> MNINDNLSINSPVDNKNVVVVRARKTDTVFKAFKVAPNIWVAPERYYGESLSIDEEYKVDGGIYDSNFLSQDSEKDKFLQAIITLLKRINSTNAGEKLLSLISTAIPFPYGYIGGGYYAPNMITFGSAPKSNKKLNSLISSTIPFPYAGYRETNYLSSEDNKSFYASNIVIFGPGANIVENNTVFYKKEDAENGMGTMTEIWFQPFLTYKYDEFYIDPAIELIKCLIKSLYFLYGIKPSDDLVIPYRLRSELENIEYSQLNIVDLLVSGGIDPKFINTDPYWFTDNYFSNAKKVFEDHRNIYETQIEGNNAIGNDIKLRLKQKFRININDIWELNLNYFSKEFSIMMPDRFNNALKHFYRKQYYKIDYPENYSINGFVNGQINVQLSLSDRNQDIINKPEEIINLLNGNNVSLMRSNIYGDGLKSTVDDFYSNYKIPYNRAYEYHFNNSNDSSLDNVNIGVIDNIPEIIDVNPYKENCDKFSPVQKITSTREINTNIPWPINYLQAQNTNNEKFSLSSDFVEVVSSKDKSLVYSFLSNVMFYLDSIKDNSPIDTDKKYYLWLREIFRNYSFDITATQEINTDCGINKVVTWFGKALNILNTSDSFVEEFQNLGPISLINKKENLSMPIIEIYGIPNDMLGLPLNDLNEKLFNIYLKNILYFKKVYFNFLDQWWTEYYSQYFDLICMAKQSILAQEKLIKQIIQNKLQDLFKADISMDKLNLMNLATEKTFIDLSNESQIAINNINDFLNKSAICVFDTNIYPKFISFMEQCINSVNSNVTAFIQKCTNITEDEKLQLIKLNTFMNIDFEFFDIQSIKDLITSETDLIKEEKESDYNLFLFTLQEDNNKVIEDISGKNTLVKYSDSISLVYGVNGDALYLKEPDESVSFSNKAFENGLTNSFSICFWLRNLGEDIITSKLIENKADNCGWEIYFENNGLVFSIVDCNGNEENIYLSDVISKNWYYISISIDRLRNQLLIFINDKLIANQSIEQILNIYSSNTISLVNENNPIYIEGLSILNRSITSEEVVNNYFSYLNNSYIRDISGERLEYNKTYELYNYVFPENSLYEVTENNNIYLSIKDTNNLNIQGAKFKLINIDANKQYVQKWDEGVVCLLGDEEKYVDISSENNRIQLVNSKDTAKRIIFNNDIFMPNCLTFAYNNKYLSLSLRDRNYNWMIC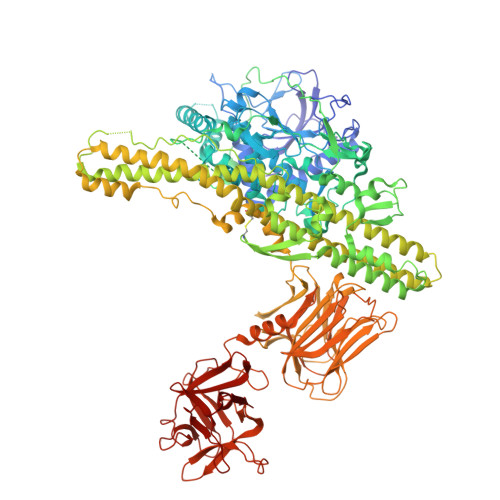NNNDNIPKAAHLWALKGI> MHHHHHHMKSIDEQS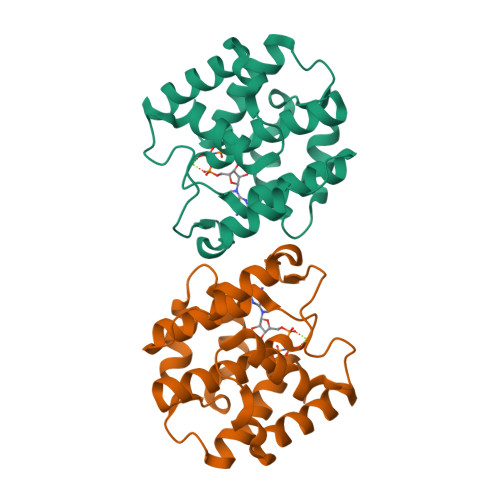LHNARRLFESGDIDRIEVGTTAGLQQIHRYLFGGLYDFAGQIREDNISKGGFRFANAMYLKEALVKIEQMPERTFEEIIAKYVEMNIAHPFLEGNGRSTRIWLDLVLKKNLKKVVNWQNVSKTLYLQAMERSPVNDLELRFLLKDNLTDDVDNREIIFKGIEQSYYYGGYEKG>[2x]GSAMADIGAEIKQGIREVILCKDQDGKIGLRLKSVDNGIFVQL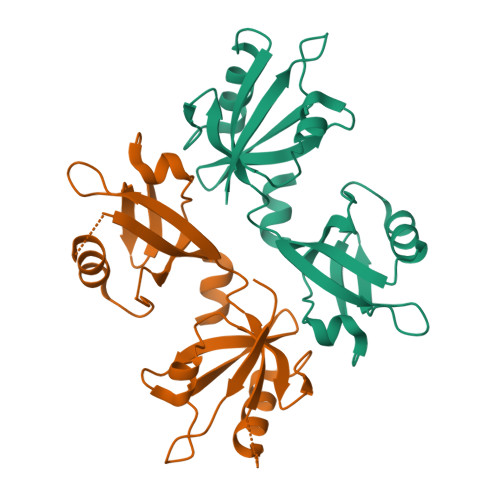VQANSPASLVGLRFGDQVLQINGENCAGWSSDKAHKVLKQAFGEKITMTIRDRPFERTVTMHKDSSGHVGFIFKSGKITSIVKDSSAARNGLLTDHHICEINGQNVIGLKDAQIADILSTAGTVVTITIMPAFIFEHIIKRMAPSIMKSLMDHTIPEV>[4x]RKPKTGILMLNMGGPETLGDVHDFLLRLFLDRDLMTLPIQNKLAPFIAKRRTPKIQEQYRRIGGGSPIKIWTSKQGEGMVKLLDELSPNTAPHKYYIGFRYVHPLT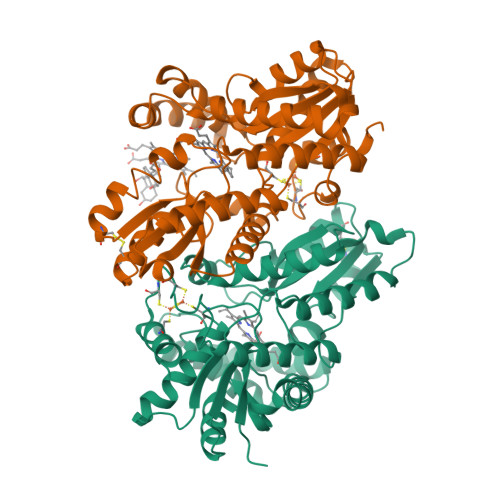EEAIEEMERDGLERAIAFTQYPQYSCSTTGSSLNAIYRYYNQVGRKPTMKWSTIDRWPTHHLLIQCFADHILKELDHFPLEKRSEVVILFSAHSLPMSVVNRGDPYPQEVSATVQKVMERLEYCNPYRLVWQSKVGPMPWLGPQTDESIKGLCERGRKNILLVPIAFTSDHIKTLYELDIEYSQVLAKECGVENIRRAESLNGNPLFSKALADLVHSHIQSNELCSKQLTLSCPLCVNPVCRETKSFFTSQQL> MLTRLAALGRPAVLDAAAAAVVVAVEPSASASAAWRDGGRDASTSYGVHSLPLAWGAQRRALGALASGCASTAPTPMVASAASAAAQARTGLPFSTAASTPAPVNAPPPPVNAPHLSNTPAELEEAELAGLDMESLMRAIVHPLPLGRVRNGALLAQALGTGAPVVQLENGPGGRDAALFFDPAATLSSTMRALHVIRQVLEKDGHVVVVNSNPRMRPLLREAAHLCLNSNVWFWADDWLPGCLAETDARGGHCPLLSDKAQPNRQIMAEKGLVFRNPLVPDRGNPAAVLGGPAPRLSAADMQRLLAGARSPMGLTHSVYKREQTASHRGCRKALAALTAARTAEARLLLPGSQTGAGRGRFRQPALVVVLDLSYGGEAVREAAARNVPTV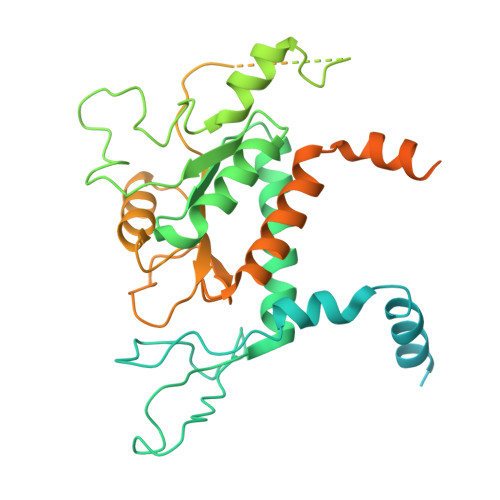ALLNGHSDASAVTFPVYASESHLGYHHFFLEWLLRVVNIDPKVLHTLRNAARAAPSAGATGATGATGATGATGATGATGATGATGATGATGATGATGATGATGARAAHAGAGAGAAAAPAAGSGKAAGKAGQQGGRGKR> MTMAANTDRAVLQ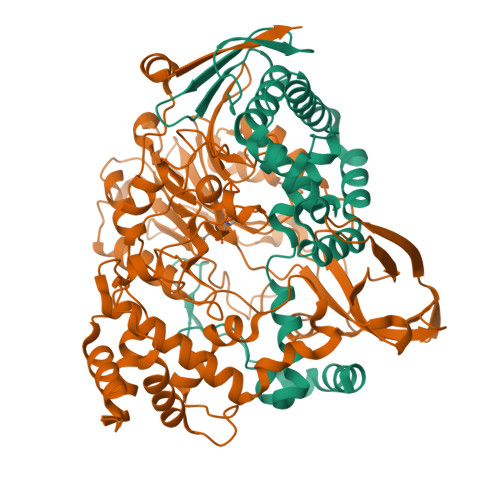AALPPLSGSLPIPGLSASVRVRRDAWGIPHIKASGEADAYRALGFVHSQDRLFQMELTRRKALGRAAEWLGAEAAEADILVRRLGMEKVCRRDFEALGVEAKDMLRAYVAGVNAFLASGAPLPVEYGLLGAEPEPWEPWHSIAVMRRLGLLMGSVWFKLWRMLALPVVGAANALKLRYDDGGRDLLCIPPGAEADRLEADLATLRPAVDALLKAMG;> SNNWAVAPGRTATGRPILAGDPHRVFEIPGFYAQHHLACDRFDMIGLTVPGVPGFPHFAHNGKVAYCVTHAFMDIHDLYLEQFAGEGRTARFGNDFEPVAWSRDRIAVRGGADREFDIVETRHGPVIAGDPRDGAALTLRSVQFAETDLSFDCLTRMPGASTVAQLYDATRGWGLIDHNLVAGDVAGSIGHLVRARVPSRPRENGWLPVPGWSGEHEWRGWIPHEAMPRVIDPPGGIIVTANNRVVADDHPDYLCTDCHPPYRAERIMKRLVANPAFAVDDAAAIHADTLSPHVGLLRRRLEALGARDDSAAEGLRQMLVAWDGRMDAASEVASAYNAFRRALTRLVTDRSGLEQAISHPFAAVAPGVSPQGQVWWAVPTLLRDDDAGMLKGWSWDQALSEALSVASQNLTGRSWGEEHRPRFTHPLATQFPAWAGLLNPASRPIGGDGDTVLANGLVPSAGPQATYGALSRYVFDVGNWDNSRWVVFHGASGHPASAHYADQNAPWSDCAMVPMLYSWDRIAAEAVTSQELVPALEHHHHHH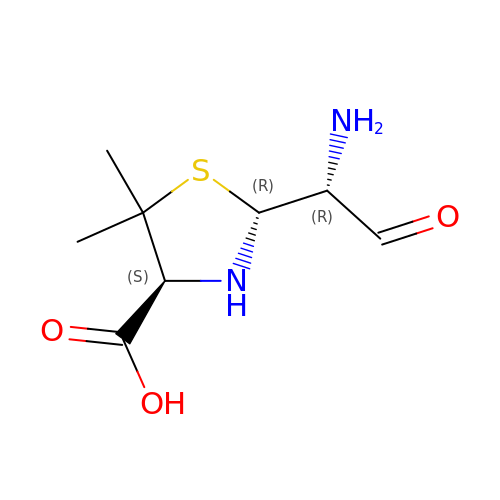(2R,4S)-2-[(1R)-1-amino-2-oxoethyl]-5,5-dimethyl-1,3-thiazolidine-4-carboxylic acid | C8 H14 N2 O3 S | SVTWYXMNISTMAS-NGJCXOISSA-N>SIKEMPFITCDEFNGVPSYMKSRLTYNQINDVIKEINKAVISKYKILHQPKKSMNSVTRNLYHRFIDEETKDTKGRYFIVEADIKEFTTLKADKKFHVLLNILRHCRRLSEVRGGGLTRYVIT[2x]

Originally discovered in a proteomics screen, the Ska complex is now recognized as a key element required for maintaining stable KT–MT attachments. The ternary Ska complex, composed of Ska1, Ska2 and Ska3, localizes to the outer KT in a KMN-dependent manner. Although GST–Ska1133–255 is not strictly equivalent to the FL Ska1 dimer in the native complex, and thus might bind MTs differently, it clearly interacted with MTs more efficiently than Ska1133–255. These observations suggest that Ska1133–255 (from now on referred to as MTBD) is the major MT-binding element within the Ska complex, which, on dimerization, can bind MTs more efficiently. Here we have used biochemical and high-resolution structural analysis to show that the human Ska complex interacts with MTs through the C-terminal domain of Ska1, which forms a variant form of winged-helix domain.

To understand the structural basis for the ability of human Ska complex to bind MTs, we obtained crystals of the Ska1–MTBD in two different crystal forms that diffracted X-rays to about 2 Å. Models from crystal form I (space group C2221) and II (space group P32) were refined to 2.1 and 2.3 Å with R factors of 19.6 and 22.5, and Rfree factors of 25.1 and 26.8, respectively, and superpose well with an overall root mean square deviation of 0.6 Å. Residues 133–142 are stabilized in an extended conformation, followed by eight α-helical segments (α1–α8) and a C-terminal β-hairpin. The structural analysis showed that the Ska1–MTBD is related to a winged-helix domain, a domain known for its ability to bind DNA and in mediating protein–protein interactions. The Ska1–MTBD differs from the canonical winged-helix domain by the incorporation of two additional modules. Analysis of the electrostatic surface potential revealed the existence of contiguous positively charged patches all over the Ska1–MTBD surface, suggesting the potential involvement of multiple MT contact sites. Although mutations at K170/177 and K135/203/206 showed no major effects on MT binding, mutations at R155/236/245, a region reported recently to be critical for MT binding, together with two new regions identified in this study, K183/184/203/206 and K217/223/226/227, all showed significant reductions in MT binding (Kd=20±4.5, 17.1±5.5 and 14.5±2.8 μM, respectively, versus WT=2.9±0.6 μM), pointing to the existence of multiple MT interaction sites. Confirming this notion, a combination of R236/245A with R155A resulted in stronger reduction in MT binding than R236/245A alone, and the simultaneous mutation of multiple clusters (K183/184/203/206/217/223/226/227/R236/245A) almost completely abolished MT binding. These results provide clear evidence that the human Ska complex binds MTs through a multipartite binding mode of Ska1–MTBD. Remarkably, the tubulin contact sites are dispersed across the surface of the Ska1–MTBD and distances between different contact sites range between 15 and 30 Å.> SEELEKALSKLSEREAMVLKMRKGLIDGREHTLEEV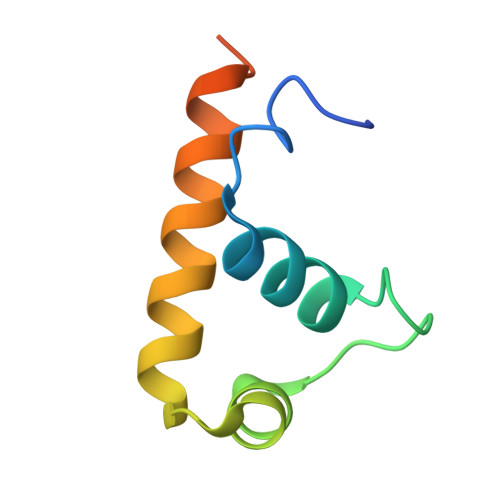GAYFGVTRERIRQIENKALRKLKYHESRTRKLRDFLE>MPGLRVPERRFSRVLGVGSYRPRREVSNKEVCTWIDSTEEWIETRTGIRSRRIAEPDETIQVMGVAASRRALEHAGVDPAEIDLVVVSTMTNFVHTPPLSVAIAHELGADNAGGFDLSAACAGFCHALSIAADAVESGGS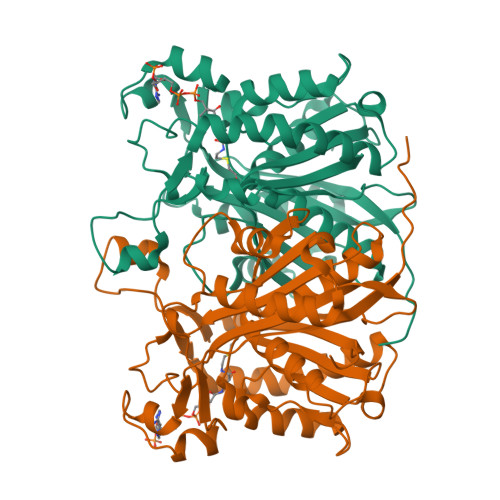RHVLVVATERMTDVIDLADRSLSFLFGDGAGAAVVGPSDVPGIGPVVRGIDGTGLGSLHMSSSWDQYVEDPSVGRPALVMDGKRVFRWAVADVVPAAREALEVAGLTVGDLVAFVPHQANLRIIDVLVDRLGVPEHVVVSRDAEDTGNTSSASVALALDRLVRSGAVPGGGPALMIGFGAGLSYAGQALLLPDPPSTPA[2x]> MRGSHHHHHHGSMAGLGHPAAFGRATHAVVRALPESLGQHALRSAKGEEVDVARAERQHQLYVGVLGSKLGLQVVELPADESLPDCVFVEDVAVVCEETALITRPGAPSRRKEVDMMKEALEKLQLNIVEMKDENATLDGGDVLFTGREFFVGLSKRTNQRGAEILADTFKDYAVSTVPVADGLHLKSFCSMAGPNLIAIGSSESAQKALKIMQQMSDHRYDKLTVPDDIAANCIYLNIPNKGHVLLHRTPEEYPESAKVYEKLKD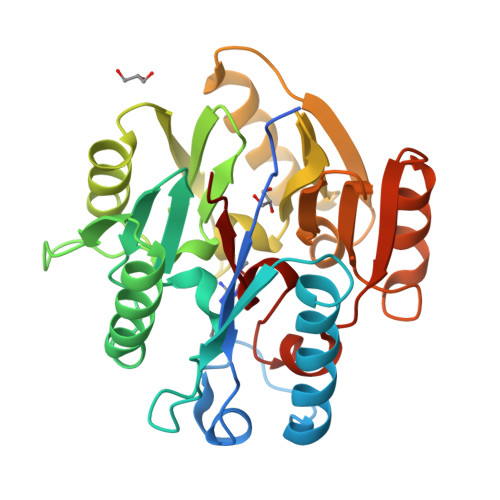HMLIPVSMSELEKVDGLLTCCSVLINKKVDS> METGNKYIEKRAIDLSRERDPNFFDNPGIPVPECF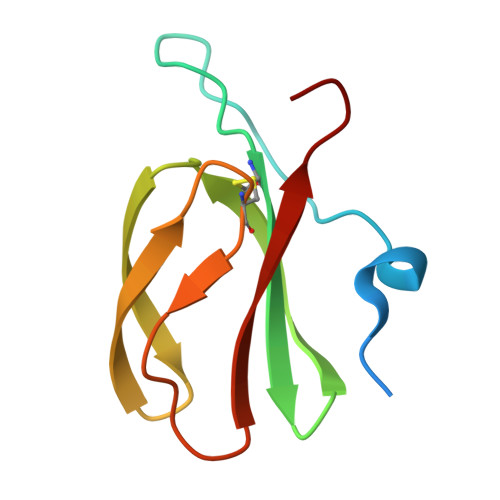WFMFKNNVRQDAGTCYSSWKMDMKVGPNWVHIKSDDNCNLSGDFPPGWIVLGKKRPGF> GSHMSQTEPPEDLMQYEAMAQDALRGVVKAALKKAAAPGGLPEPHHLYITFKTKAAGVSGPQDLLSKYPDEMTIVLQHQYWDLAPGETFFSVTLKFGGQPKRLSVPYAA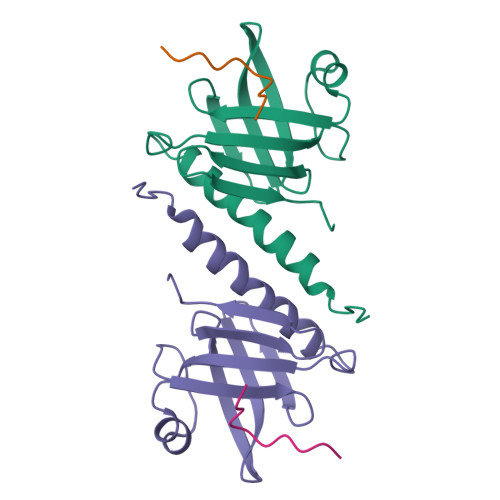LTRFYDPSVQFALQFSAPEIIEDEPEPDPEPEDKANQGASGDEGPKIV;> KKGRHGAANDNFAEEFAVAA>[2x]GSASTVKGSVDLEKLAFGLTKLNEDDLVGVVQMVTDNKTPEMNVTNNVEEGEFIIDLYSLPEGLLKSLWDYVKKNT;>SRSFMVKIRTKN[2x]

TFIIF is involved in the recruitment of RNA Pol II and the association with Mediator, whereas TFIID is responsible for binding to the promoter. Both yeast TFIID and TFIIF contain multiple subunits and share one subunit – Taf14 (transcription initiation factor subunit 14). Taf14 is a 244-residue protein, which consists of the N-terminal YEATS (Yaf9, ENL, AF9, Taf14, Sas5) domain and the extra-terminal (ET) domain. The YEATS domain of Taf14 recognizes acylated lysine 9 of histone H3 (H3K9acyl), and the ET domain is capable of associating with the hxhKh motif found in several co-activators, such as Sth1 and Taf213. Here, we determined the molecular and structural basis by which the YEATS and ET domains of Taf14 bind to the C-terminal tail of Taf2 and identified a unique DNA-binding activity of the linker region connecting the two domains.

The slow exchange regime on the NMR timescale suggested tight binding, which was confirmed by measuring binding affinity of Taf14ET for Taf2CT using MST (the dissociation constant (Kd) = 1.6 μM). To gain insight into the binding mechanism, we crystallized the Taf14ET-Taf2CT complex and determined its structure to 1.7 Å by X-ray crystallography. Taf14ET adopts a three-helix bundle fold with a two-stranded anti-parallel β-sheet connecting helices α2 and α3. The Taf2CT peptide is in an extended conformation and occupies an elongated, primarily hydrophobic groove of Taf14ET. Taf2CT pairs with the second β-strand of Taf14ET, forming the third anti-parallel β-strand in the β-sheet, and makes extensive intermolecular contacts with the domain. Characteristic β-sheet interactions are observed between the backbone amides of V1397, I1399 and T1401 of Taf2CT and G218, F220 and I222 of Taf14ET. The side chains of V1397 and I1399 of Taf2CT are oriented toward and essentially buried in the hydrophobic groove of Taf14ET. The complex is further stabilized by a set of additional hydrogen bonds formed between the backbone amide group of F1395 of Taf2CT and the side chain carboxyl group and the backbone amino group of D223 of Taf14ET. The side chain amino group of K1398 of Taf2CT donates a transient hydrogen bond to the side chain carboxyl moiety of E219 of Taf14ET, whereas the guanidino moiety of R1400 of Taf2CT is hydrogen bonded to the backbone carbonyl group of K1398. In the Taf14ET-Taf2CT complex, the only lysine residue of Taf2CT, K1398, is in the middle of the β-strand and thus its position is fixed.> GAMGMTNPFENKEGTYLVLINDEGQYSLWPASIAIPPGW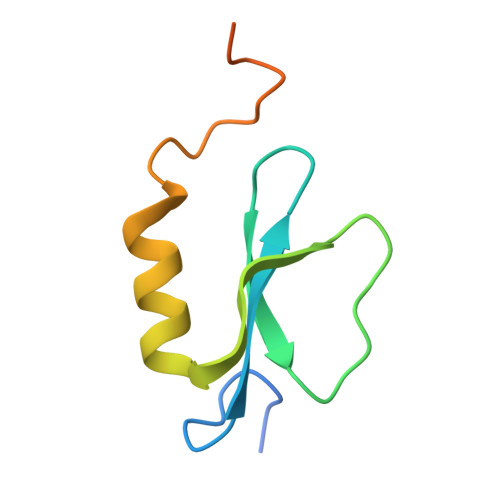NIAFAENTRSACLDYINAHWIDMRPNSLKDGSLSKRDNDYSGVK>MKEDLNLRLKKLTHAAPCMLFMKGTPQEPRCGFSKQMVEILHKHNIQFSSFDIFSDEEVRQGLKAYSSWPTYPQLYVSGELIGGLDIIKELEASE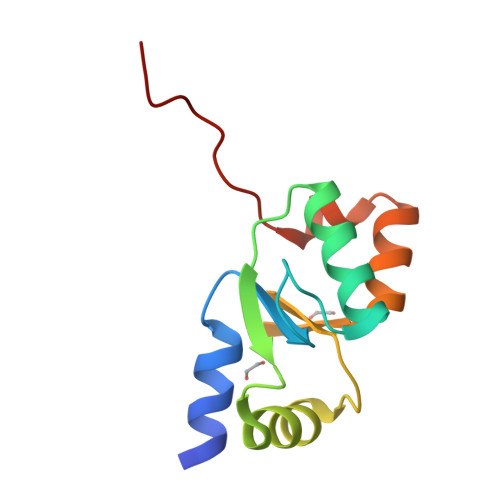ELDTICPKAAENLYFQ[2x]> GPPGEVMGRAIARVADTIGSGPVNSESIPALTAAETGHTSQVVPSDTMQTRHVKNYHSRSESTVENFLCRSACV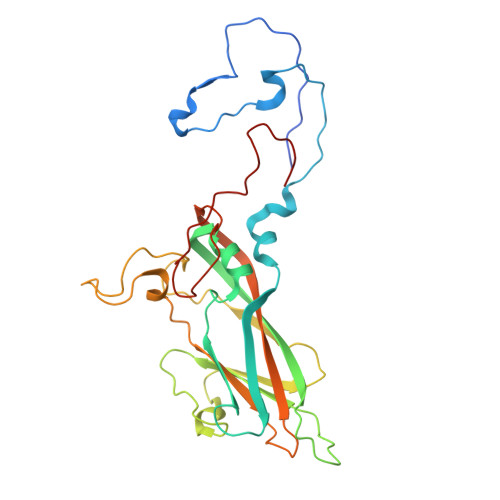FYTTYENHDSDGDNFAYWVINTRQVAQLRRKLEMFTYARFDLELTFVITSTQEQPTVRGQDAPVLTHQIMYVPPGGPVPTKVNSYSWQTSTNPSVFWTEGSAPPRMSVPFIGIGNAYSMFYDGWARFDKQGTYGISTLNNMGTLYMRHVNDGGPGPIVSTVRIYFKPKHVKTWVPRPPRLCQYQKAGNVNFEPTGVTEGRTDITTMKTT> GAMGRILFLTTFMSKGNKVVRYLESLHHEVVICQEKVHAQSANLQEIDWIVSYAYGYILDKEIVSRFRGRIINLHPSLLPWNKGRDPVFWSVWDETPKGVTIHLIDEHVDTGDILVQEEIAFADEDTLLDCYNKANQAIEELFIREWENIVHGRIAPYRQTAGGTLHFKADRDFYKNLNMTTVRELLALKRLCAEPKRGEKPIDKTFHQLFEQQVEMTPDHVAVVDRGQSLTYKQLNERANQLAHHLRGKGVKPDDQVAIMLDKSLDMIVSILAVMKAGGAYVPIDPDYPGERIAYMLADSSAAILLTNALHEEKANGACDIIDVHDPDSYSENTNNLPHVNRPDDLVYVMYTSGSTGLAKGVMIEHHNLVNFCEWYRPYFGVTPADKALVYSSFSFDGSALDIFTHLLAGAALHIVPSERKYDLDALNDYCNQEGITISYLPTGAAEQFMQMDNQSFRVVITGGDVLKKIERNGTYKLYNGYGMTECTIMVTMFEVDKPYANIPIGKPIDRTRILILDEALALQPIGVAGELFIVGEGLGRGYLNRPELTAEKFIVHPQTGERMYRTGDRARFLPDGNIEFLGRLDNLVKIRGYRIEPGEIEPFLMNHPLIELTTVLAK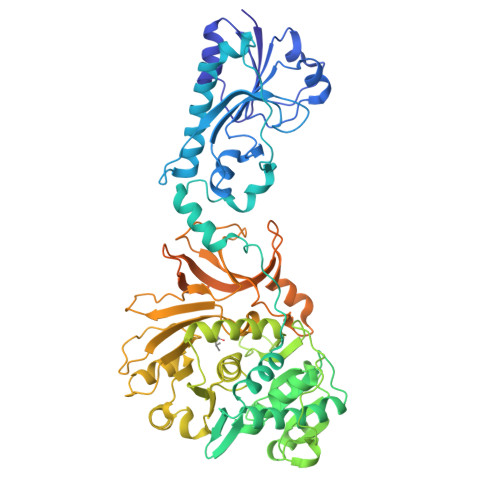EQADGRKYLVGYYVAPEEIPHGELREWLGNDLPDYMIPTYFVHMKAFPLTANGKVDRRALPDVQADA> MEPRVGNKFRLGRKIGSGSFGEIYLGTNIQTNEEVAIKLENVKTKHPQLLYESKIYRILQGGTGIPNVRWFGVEGDYNVLVMDLLGPSLEDLFNFCSRKLSLKTVLMLADQMINRVEFVHSKSFLHRDIKPDNFLMGLGRRANQVYIIDFGLAKKYRDTSTHQHIPYRENKNLTGTARYASVNTHLGIEQSRRDDLESLGYVLMYFLRGSLPWQGLKAG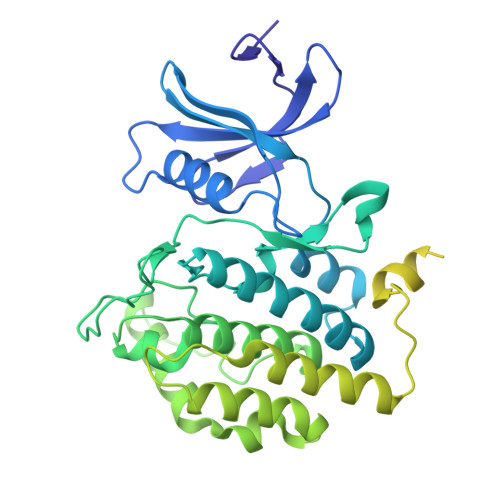TKKQKYEKISEKKVATSIEALCRGYPTEFASYFHYCRSLRFDDKPDYSYLKRLFRDLFIREGFQFDYVFDWTILKYQQSQIASAPPRAVGHGAGPSGLAPPALQNDRQSGVDEGRTSGWSSMDRRRAPPPIASVGTLAKQKAPVGNDASFSKEPVISASNFLGRSSGSSRRPAVSSSRDVMPIDTSEPSRTRATDASPGAFRRTSGPQKSSPVNSAEPKHSSSARHSSNVKNYESALKGIEGLNFDGDERVQYAAALEHHHHHH>[2x]NVFTAQNTAQDFNGNESTVKSFYVTRTGKKILVAITSTKDNLKTVTCLTETGKTVLNL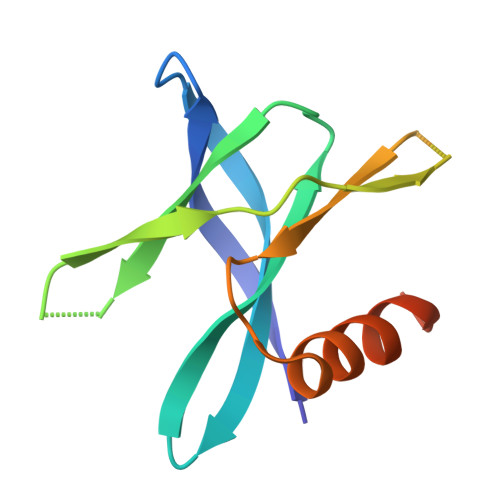DPPMRFAHTVGGKQSVVYLYFIQNISSLNRGMVIGHISETTILQHHHHHH(1S,3S)-3-methylcyclohexan-1-ol | C7 H14 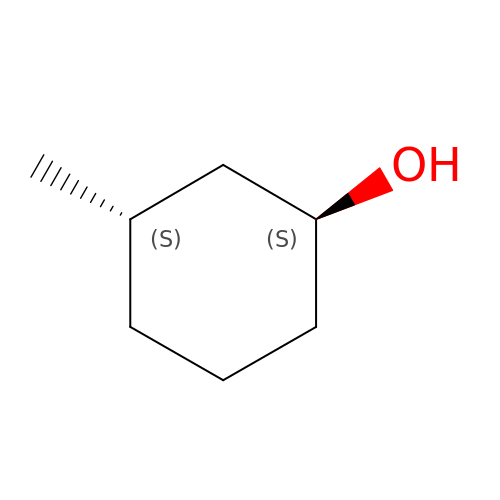O | HTSABYAWKQAHBT-BQBZGAKWSA-N>RLKALQQKQTQTTSAAEDKTKPLEEAFDWDEYPVQRVTATGYTAGAES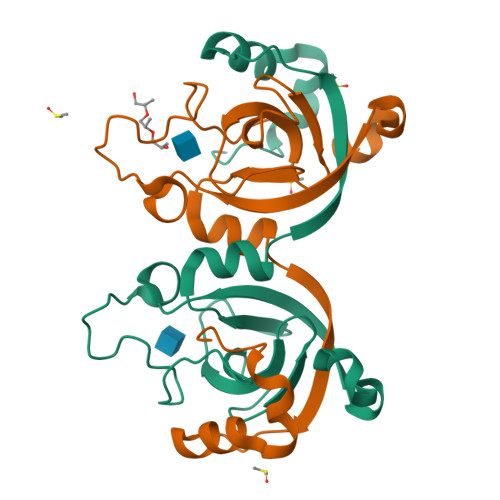TGKNPGDPLYGLTYSGVKVKRDLYSTVAADPSVFPIGTILFIPNYGLGVVADTGSAIKGNRLDLYFETVKDVYNEWGKKTLDVYVIKKGTGKITEDELEKLNETKSLQVFRNQYKTVKE[2x]> QGGDRVKKLINSQISLLIGKGLHEFDSLRDPEVNDFRTKMRQFCEEAAAHRQQLGWVEWLQYSFPLQLEPSARGWRAGLLRVSNRALLVNVKFEGSEESFTFQVSTKDMPLALMACALRKKATVFRQPLVEQPEEYALQVNGRHEYLYGNYPLCHFQYICSCLHSGLTPHLTMVHSSSILAMRDEQSNPAPQVQKPRAKPPPIPAKKPSSVSLWSLEQPFSIELIEGRKVNADERMKLVVQAGLFHGNEMLCKTVSSSEVNVCSEPVWKQRLEFDISVCDLPRMARLCFALYAVVEKAKKARSTKKKSKKADCPIAWANLMLFDYKDQLKTGERCLYMWPSVPDEKGELLNPAGTVRGNPNTESAAALVIYLPEVAPHPVYFPALEKILELGRHGERGRITEEEQLQLREILERRGSGELYEHEKDLVWKMRHEVQEHFPEALARLLLVTKWNKHEDVAQMLYLLCSWPELPVLSALELLDFSFPDCYVGSFAIKSLRKLTDDELFQYLLQLVQVLKYESYLDCELTKFLLGRALANRKIGHFLFWHLRSEMHVPSVALRFGLIMEAYCRGSTHHMKVLMKQGEALSKLKALNDFVKVSSQKTTKPQTKEMMHMCMRQETYMEALSHLQSPLDPSTLLEEVCVEQCTFMDSKMKPLWIMYSSEEAGSAGNVGIIFKNGDDLRQDMLTLQMIQLMDVLWKQEGLDLRMTPYGCLPTGDRTGLIEVVLHSDTIANIQLNKSNMAATAAFNKDALLNWLKSKNPGEALDRAIEEFTLSCAGYCVATYVLGI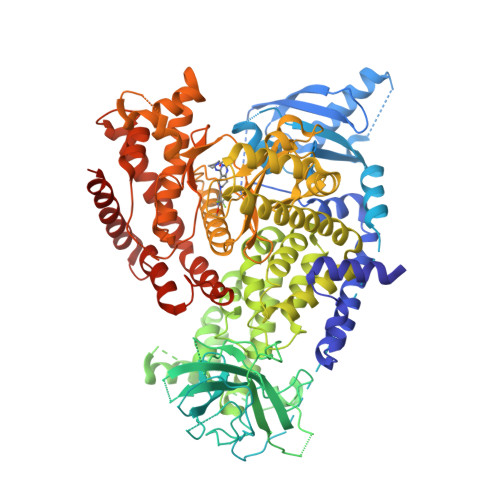GDRHSDNIMIRESGQLFHIDFGHFLGNFKTKFGINRERVPFILTYDFVHVIQQGKTNNSEKFERFRGYCERAYTILRRHGLLFLHLFALMRAAGLPELSCSKDIQYLKDSLALGKTEEEALKHFRVKFNEALRESWKTKVNWLAHNVSKDNRQ>[2x]MKHSFSRFFGLGEKEQEPEIAEHDTNKEEILEIPVNAIVPNRFQPRTIFSDEKIKELAMTIHTHGIIQPIVVRHTEEEGQYELIAGERRWRAVQSLEWEKIPAIIKDFSDTETASVALIENLQREELSSIEEAHAYARLLELHDLTQEALAQR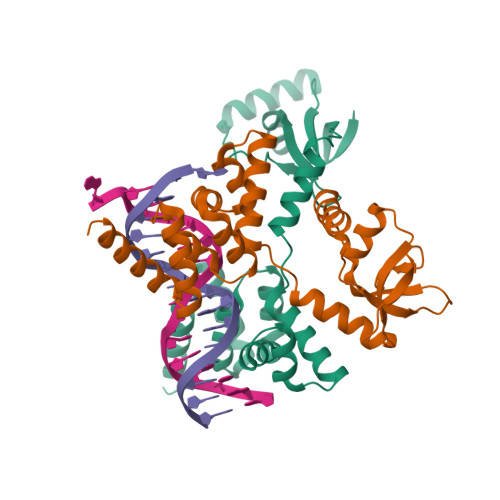LGKGQSTIANKLRLLKLPQPVQEAIMEKKITERHARALIPLKQPELQVTLLTEIIEKSLNVKQTEDRVVKMLEQGQRKPKPRRKAFSRDKLAAALEHHHHHH> A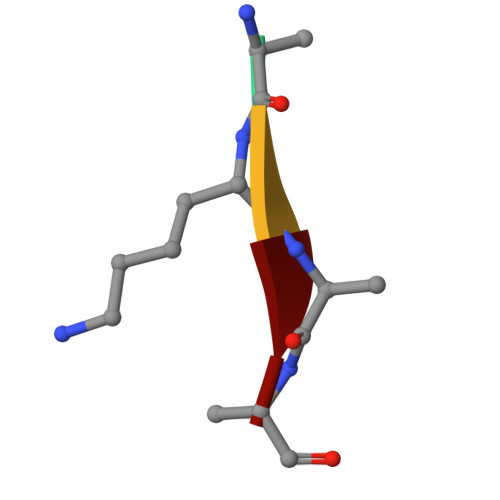KAA>[3x]SNKKQSNRLTEQHKLSQGVIGIFGDYAKAHDLAVGEVSKLVKKALSNEYPQLSFRYRDSIKKTEINEA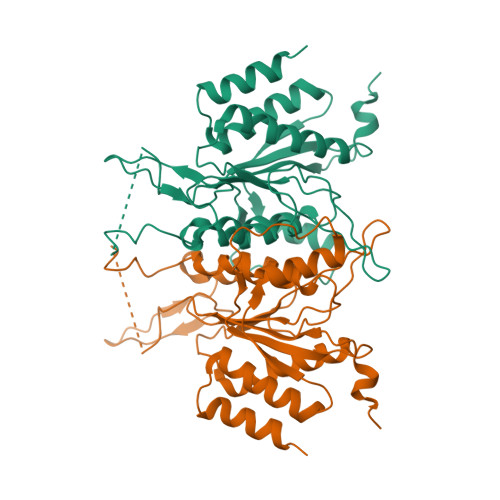LKKIDPDLGGTLFVSNSSIKPDGGIVEVKDDYGEWRVVLVAEAKHQGKDIINIRNGLLVGKRGDQDLMAAGNAIERSHKNISEIANFMLSESHFPYVLFLEGSNFLTENISITRPDGRVVNLEYNSGILNRLDRLTAANYGMPINSNLCINKFVNHKDKSIMLQAASIYTQGDGREWDSKIMFEIMFDISTTSLRVLGRDLFEQLTSK> SMQGPRTRPRKPIRCGEVLFAVGGWCSGDAISSVERYDPQTNEWRMVASMSKRRCGVGVSVLDDLLYAVGGHDGSSYLNSVERYDPKTNQWSSDVAPTSTCRTSVGVAVLGGFLYAVGGQDGVSCLNIVERYDPKENKWTRVASMSTRRLGVAVAVLGGFLYAVGGSDGTSPLNTVERYNPQENRWHTIAPMGTRRKHLGCAVYQDMIYAVGGRDDTTELSSAERYNPRTNQWSPVVAMTSRRSGVGLAVVNGQLMAVGGFDGTTYLKTIEVFDPDANTWRLYGGMNYRRLGGGVGVIKMTHCE;> LGLPDLVAKYN

Kelch-like protein 20 (KLHL20, also known as KLEIP) is a member of the BTB-Kelch family that assembles with CUL3 and RBX1 to form a multi-subunit Cullin-RING E3 ligase (Geyer et al., 2003, Hara et al., 2004, Pintard et al., 2004). The BTB and 3-box domains confer binding to CUL3, whereas the Kelch β-propeller domain serves as the substrate recognition domain (Canning et al., 2013, Lee et al., 2010). KLHL20 is a related CUL3-dependent ubiquitin ligase linked to autophagy, cancer, and Alzheimer's disease that promotes the ubiquitination and degradation of substrates including DAPK1, PML, and ULK1. Here, we investigated the binding of KLHL20 to DAPK1, which was the first reported substrate for this E3 ligase (Lee et al., 2010).

For further co-crystallization trials, we tried an 11-residue DAPK1 peptide (LGLPDLVAKYN) in order to capture interactions of the central “LPDLV” motif, while allowing for local conformational preferences and potential flanking interactions. The structure was refined at 1.1-Å resolution and traced the full KLHL20 Kelch domain from residues 317 to 601. The Kelch domain structure shows a canonical β-propeller fold. The bound DAPK1 peptide shows an extended conformation that packs between Kelch domain blades II and III at its N terminus and blades V and VI at its C terminus. At its center, the peptide adopts a single loose helical turn that is stabilized by intramolecular hydrogen bonds between the carbonyl of Pro1337 and the amides of Val1340 and Ala1341. Here, the peptide inserts deeply into the central cavity of the Kelch domain β propeller where it is anchored in the complex by Leu1339, the second leucine in the “LPDLV” motif. The “LPDLV” motif of DAPK lies at the core of the protein-peptide interface. Here, the hydrophobic side chains pack against Kelch domain blades I and II and make notable van der Waals contacts with KLHL20 Trp326, His373, and Leu592, respectively. By contrast, the second leucine, Leu1339, is the most buried DAPK1 residue in the complex. The final residue in the “LPDLV” motif, DAPK1 Asp1338, is oriented away from the hydrophobic side chains to face Kelch domain blade V, where it forms a salt bridge with KLHL20 Lys498 as well as a hydrogen bond to His499.> MAAEEGVASAASAGGSWGTAAMGRVLPMLLVPVPAEAMGQLGSRAQLRTQPEALGSLTAAGSLQVLSLTPGSRGGGRCCLEGPFWHFLWEDSRNSSTPTEKPKLLALGENYELLIYEFNLKDGRCDATILYSCSREALQKLIDDQDISISLLSLRILSFHNNTSLLFINKCVILHIIFPERDAAIRVLNCFTLPLPAQAVDMIIDTQLCRGILFVLSSLGWIYIFDVVDGTYVAHVDLALHKEDMCNEQQQEPAKISSFTSLKVSQDLDVAVIVSSSNSAVALNLNLYFRQHPGHLLCERILEDLPIQGPKGVDEDDPVNSAYNMKLAKFSFQIDRSWKAQLSSLNETIKNSKLEVSCCAPWFQDILHLESPESGNHSTSVQSWAFIPQDIMHGQYNVLQKDHAKTSDPGRSWKIMHISEQEEPIELKCVSVTGFTALFTWEVERMGYTITLWDLETQGMQCFSLGTKCIPVDSSGDQQLCFVLTENGLSLILFGLTQEEFLNRLMIHGSASTVDTLCHLNGWGRCSIPIHALEAGIENRQLDTVNFFLKSKENLFNPSSKSSVSDQFDHLSSHLYLRNVEELIPALDLLCSAIRESYSEPQSKHFSEQLLNLTLSFLNNQIKELFIHTEELDEHLQKGVNILTSYINELRTFMIKFPWKLTDAIDEYDVHENVPKVKESNIWKKLSFEEVIASAILNNKIPEAQTFFRIDSHSAQKLEELIGIGLNLVFDNLKKNNIKEASELLKNMGFDVKGQLLKICFYTTNKNIRDFLVEILKEKNYFSEKEKRTIDFVHQVEKLYLGHFQENMQIQSFPRYWIKEQDFFKHKSVLDSFLKYDCKDEFNKQDHRIVLNWALWWDQLTQESILLPRISPEEYKSYSPEALWRYLTARHDWLNIILWIGEFQTQHSYASLQQNKWPLLTVDVINQNTSCNNYMRNEILDKLARNGVFLASELEDFECFLLRLSRIGGVIQDTLPVQNYKTKEGWDFHSQFILYCLEHSLQHLLYVYLDCYKLSPENCPFLEKKELHEAHPWFEFLVQCRQVASNLTDPKLIFQASLANAQILIPTNQASVSSMLLEGHTLLALATTMYSPGGVSQVVQNEENENCLKKVDPQLLKMALTPYPKLKTALFPQCTPPSVLPSDITIYHLIQSLSPFDPSRLFGWQSANTLAIGDAWSHLPHFSSPDLVNKYAIVERLNFAYYLHNGRPSFAFGTFLVQELIKSKTPKQLIQQVGNEAYVIGLSSFHIPSIGAACVCFLELLGLDSLKLRVDMKVANIILSYKCRNEDAQYSFIRESVAEKLSKLADGEKTTTEELLVLLEEGTWNSIQQQEIKRLSSESSSQWALVVQFCRLHNMKLSISYLRECAKANDWLQFIIHSQLHNYHPAEVKSLIQYFSPVIQDHLRLAFENLPSVPTSKMDSDQVCNKCPQELQGSKQEMTDLFEILLQCSEEPDSWHWLLVEAVKQQAPILSVLASCLQGASAISCLCVWIITSVEDNVATEAMGHIQDSTEDHTWNLEDLSVIWRTLLTRQKSKTLIRGFQLFFKDSPLLLVMEMYELCMFFRNYKEAEAKLLEFQKSLETLNTAATKVHPVIPAMWLEDQVCFLLKLMLQQCKTQYELGKLLQLFVEREHLFSDGPDVKKLCILCQILKDTSIAINHTIITSYSIENLQHECRSILERLQTDGQFALARRVAELAELPVDNLVIKEITQEMQTLKHIEQWSLKQARIDFWKKCHENFKKNSISSKAASSFFSTQAHVACEHPTGWSSMEERHLLLTLAGHWLAQEDVVPLDKLEELEKQIWLCRITQHTLGRNQEETEPRFSRQISTSGELSFDSLASEFSFSKLAALNTSKYLELNSLPSKETCENRLDWKEQESLNFLIGRLLDDGCVHEASRVCRYFHFYNPDVALVLHCRALASGEASMEDLHPEIHALLQSAELLEEEAPDIPLRRVHSTSSLDSQKFVTVPSSNEVVTNLEVLTSKCLHGKNYCRQVLCLYDLAKELGCSYTDVAAQDGEAMLRKILASQQPDRCKRAQAFISTQGLKPDTVAELVAEEVTRELLTSSQGTGHKQMFNPTEESQTFLQLTTLCQDRTLVGMKLLDKISSVPHGELSCTTELLILAHHCFTLTCHMEGIIRVLQAAHMLTDNHLAPSEEYGLVVRLLTGIGRYNEMTYIFDLLHKKHYFEVLMRKKLDPSGTLKTALLDYIKRCRPGDSEKHNMIALCFSMCREIGENHEAAARIQLKLIESQPWEDSLKDGHQLKQLLLKALTLMLDAAESYAKDSCVRQAQHCQRLTKLITLQIHFLNTGQNTMLINLGRHKLMDCILALPRFYQASIVAEAYDFVPDWAEILYQQVILKGDFNYLEEFKQQRLLKSSIFEEISKKYKQHQPTDMVMENLKKLLTYCEDVYLYYKLAYEHKFYEIVNVLLKDPQTGCCLKDMLAG;> MNHPFGKEEAASQKQLFGFFCECLRRGEWELAQACVPQLQEGQGDIPKRVEDILQALVVCPNLLRCGQDINPQRVAWVWLLVLEKWLAREKKLLPVVFRRKLEFLLLSEDLQGDIPENILEELYETLTQGAVGHVPDGNPRRESWTPRLSSEAVSVLWDLLRQSPQPAQALLELLLEEDDGTGLCHWPLQNALVDLIRKALRALQGPDSVPPGVVDAIYGALRTLRCPAEPLGVELHLLCEELLEACRTEGSPLREERLLSCLLHKASRGLLSLYGHTYAEKVTEKPPRATASGKVSPD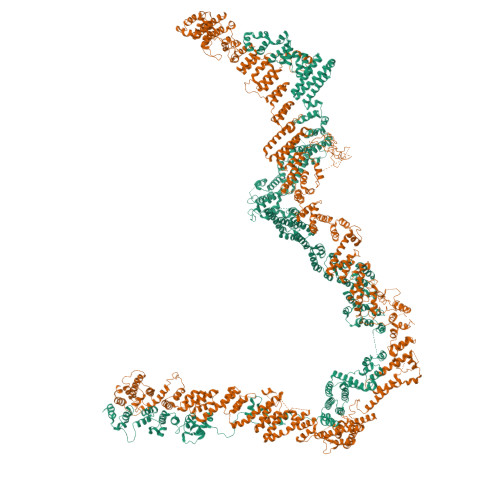HLDPERAMLALFSNPNPAEAWKVAYFYCLSNNKHFLEQILVTALTLLKEEDFPNLGCLLDREFRPLSCLLVLLGWTHCQSLESAKRLLQTLHRTQGPGCDELLRDACDGLWAHLEVLEWCIQQSSNPIPKRDLLYHLHGGDSHSVLYTLHHLTNLPALREEDVLKLLQKVPAKDPQQEPDAVDAPVPEHLSQCQNLTLYQGFCAMKYAIYALCVNSHQHSQCQDCKDSLSEDLASATEPANDSLSSPGAANLFSTYLARCQQYLCSIPDSLCLELLENIFSLLLITSADLHPEPHLPEDYAEDDDIEGKSPSGLRSPSESPQHIAHPERKSERGSLGVPKTLAYTMPSHVKAEPKDSYPGPHRHSFLDLKHFTSGISGFLADEFAIGAFLRLLQEQLDEISSRSPPEKPKQESQSCSGSRDGLQSRLHRLSKVVSEAQWRHKVVTSNHRSEEQPSRRYQPATRHPSLRRGRRTRRSQADGRDRGSNPSLESTSSELSTSTSEGSLSAMSGRNELHSRLHPHPQSSLIPMMFSPPESLLASCILRGNFAEAHQVLFTFNLKSSPSSGELMFMERYQEVIQELAQVEHKIENQNSDAGSSTIRRTGSGRSTLQAIGSAAAAGMVFYSISDVTDKLLNTSGDPIPMLQEDFWISTALVEPTAPLREVLEDLSPPAMAAFDLACSQCQLWKTCKQLLETAERRLNSSLERRGRRIDHVLLNADGIRGFPVVLQQISKSLNYLLMSASQTKSESVEEKGGGPPRCSITELLQMCWPSLSEDCVASHTTLSQQLDQVLQSLREALELPEPRTPPLSSLVEQAAQKAPEAEAHPVQIQTQLLQKNLGKQTPSGSRQMDYLGTFFSYCSTLAAVLLQSLSSEPDHVEVKVGNPFVLLQQSSSQLVSHLLFERQVPPERLAALLAQENLSLSVPQVIVSCCCEPLALCSSRQSQQTSSLLTRLGTLAQLHASHCLDDLPLSTPSSPRTTENPTLERKPYSSPRDSSLPALTSSALAFLKSRSKLLATVACLGASPRLKVSKPSLSWKELRGRREVPLAAEQVARECERLLEQFPLFEAFLLAAWEPLRGSLQQGQSLAVNLCGWASLSTVLLGLHSPIALDVLSEAFEESLVARDWSRALQLTEVYGRDVDDLSSIKDAVLSCAVACDKEGWQYLFPVKDASLRSRLALQFVDRWPLESCLEILAYCISDTAVQEGLKCELQRKLAELQVYQKILGLQSPPVWCDWQTLRSCCVEDPSTVMNMILEAQEYELCEEWGCLYPIPREHLISLHQKHLLHLLERRDHDKALQLLRRIPDPTMCLEVTEQSLDQHTSLATSHFLANYLTTHFYGQLTAVRHREIQALYVGSKILLTLPEQHRASYSHLSSNPLFMLEQLLMNMKVDWATVAVQTLQQLLVGQEIGFTMDEVDSLLSRYAEKALDFPYPQREKRSDSVIHLQEIVHQAADPETLPRSPSAEFSPAAPPGISSIHSPSLRERSFPPTQPSQEFVPPATPPARHQWVPDETESICMVCCREHFTMFNRRHHCRRCGRLVCSSCSTKKMVVEGCRENPARVCDQCYSYCNKDVPEEPSEKPEALDSSKNESPPYSFVVRVPKADEVEWILDLKEEENELVRSEFYYEQAPSASLCIAILNLHRDSIACGHQLIEHCCRLSKGLTNPEVDAGLLTDIMKQLLFSAKMMFVKAGQSQDLALCDSYISKVDVLNILVAAAYRHVPSLDQILQPAAVTRLRNQLLEAEYYQLGVEVSTKTGLDTTGAWHAWGMACLKAGNLTAAREKFSRCLKPPFDLNQLNHGSRLVQDVVEYLESTVRPFVSLQDDDYFATLRELEATLRTQSLSLAVIPEGKIMNNTYYQECLFYLHNYSTNLAIISFYVRHSCLREALLHLLNKESPPEVFIEGIFQPSYKSGKLHTLENLLESIDPTLESWGKYLIAACQHLQKKNYYHILYELQQFMKDQVRAAMTCIRFFSHKAKSYTELGEKLSWLLKAKDHLKIYLQETSRSSGRKKTTFFRKKMTAADVSRHMNTLQLQMEVTRFLHRCESAGTSQITTLPLPTLFGNNHMKMDVACKVMLGGKNVEDGFGIAFRVLQDFQLDAAMTYCRAARQLVEKEKYSEIQQLLKCVSESGMAAKSDGDTILLNCLEAFKRIPPQELEGLIQAIHNDDNKVRAYLICCKLRSAYLIAVKQEHSRATALVQQVQQAAKSSGDAVVQDICAQWLLTSHPRGAHGPGSRK>AMAPAKKSEELVAEAHNLCTLLENAIQDTVREQGNSMMNLDWSWLTE[2x];>EWGAPETLQRCLEENQELRDAIRQSNQILRERCEE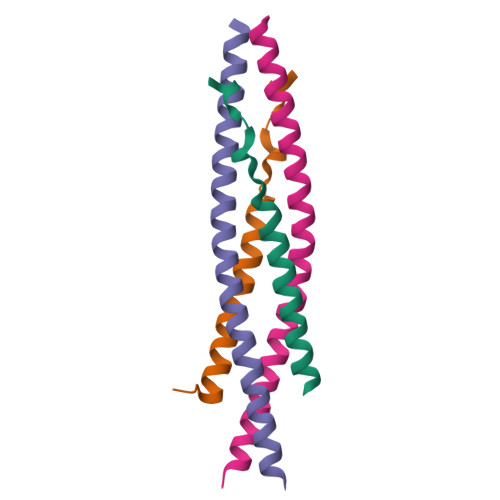LLHFQASQREEKEFLMCKFQEARKLVERLGLEK[2x]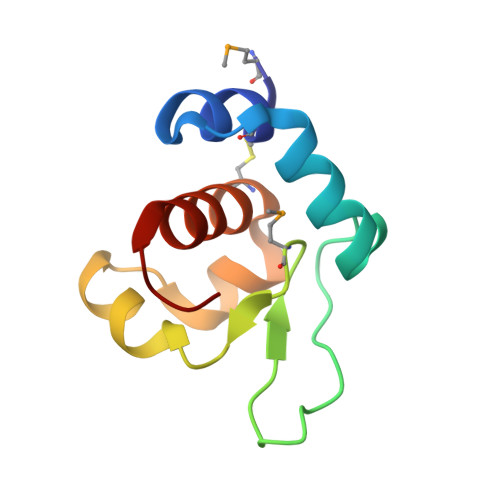> MDCFEITGKAYNIDPLILKAIAWNESKNKNGIKSKINKNGTYNIGIMQINSSHLDLLSKFNISEDDLLNDACINISVAGYILASNIKY> SADNGGYVPAVVIGTGYGAAVSALRLGEAGVQTLMLEMGQLWNQPGPDGNIFCGMLNPDKRSSWFKNRTEAPLGSFLWLDVVNRNIDPYAGVLDRVNYDQMSVYVGRGVGGGSLVNGGMAVEPKRSYFEEILPRVDSSEMYDRYFPRANSMLRVNHIDTKWFEDTEWYKFARVSREQAGKAGLGTVFVPNVYDFGYMQREAAGEVPKSALATEVIYGNNHGKQSLDKTYLAAALGTGKVTIQTLHQVKTIRQTKDGGYALTVEQKDTDGKLLATKEISCRYLFLGAGSLGSTELLVRARDTGTLPNLNSEVGAGWGPNGNIMTARANHMWNPTGAHQSSIPALGIDAWDNSDSSVFAQIAPMPA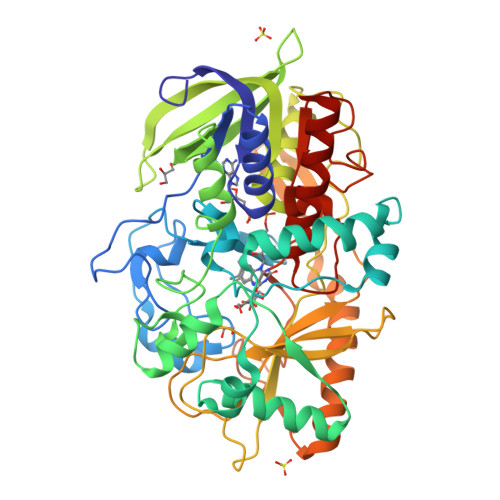GLETWVSLYLAITKNPQRGTFVYDAATDRAKLNWTRDQNAPAVNAAKALFDRINKANGTIYRYDLFGTQLKAFADDFCYQPLGGCVLGKATDDYGRVAGYKNLYVTDGSLIPGSVGVNPFVTITALAERNVERIIKQDVTAS>[2x]IREILKMGDERLLRIAQPVPSELLGSEELQRLIDDMFETMHHVGGVGLAAPQIGVDLQLVIFGFERSERYPDAPAVPPTILLNPR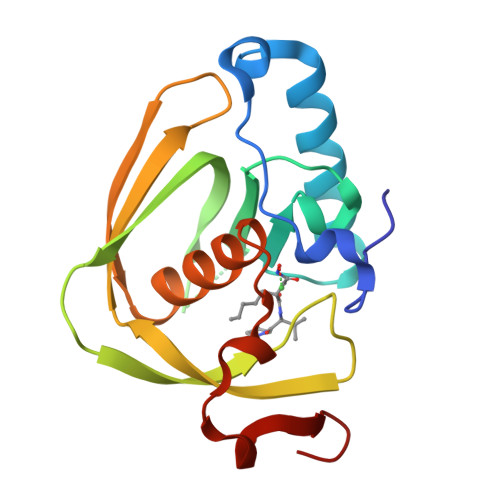ITPLDDEMEEGWEGCLSVPGLRGAVSRHRRIRYQGLDPQGQPIDRSVEGFHARVVQHECDHLIGRLYPSRITDFSKFGFTEVLF> CGNKENASNGASGKNDEKKTEQAEEMTIKHQLGEAKVKKNPEKVVVFDFGVLDTLDKLGVKVTALPQMNVPKYLEKYKSSDYQNVGSLMEPDFEKLSEIKPDVIFISGRQANLYDKLKEIGPTVYIGIDTQHYWDSFTNNMKLIGQMFGKEKEVDEELANIEKQIEEVKTKAADKKALIILTTGGKVSAYGKGSRFGLIHDVLGVPAADPNLKVTNPHGQSVSFEYIAEKNPDYLFVIDRDAVVEGKPTAKQTIENALVKKTKAYQNGHIVYLDPNYWYLSGGGLTSVSEMIKQVEEGLK

Siderophore-binding proteins from two thermophilic bacteria, Geobacillus stearothermophilus and Parageobacillus thermoglucosidasius, were identified from a search of sequence databases, cloned and overexpressed. They are homologues of the well characterized protein CjCeuE from Campylobacter jejuni. The proteins have a two-domain structure, with the domains linked by a long α-helix at the base of the fold. The siderophore binding sites sit between the two domains.

The crystal structure of apo Gst was solved by molecular replacement using the structure of CjCeuE as a search model. There is a single molecule in the asymmetric unit with a continuous chain from Met26 through to the C-terminal Lys300. The predicted and experimental apo Gst structures had an r.m.s.d. between all 273 Cα atoms of 0.62 Å. Thus, the AF2 model has accurately predicted the fold in the experimental apo structure around the ligand-binding site. In Gst and Pth, the position of the main chain of the histidine loop is closely similar in the apo, complex and predicted structures, with the histidine side chain having moved a couple of ångströms away from its iron-binding position in the apo and AF2 structures. In contrast, the histidine loop is already in the closed, iron-chelating position in the apo structures of the thermophilic proteins. It should of course be noted that these structures are from crystals cryogenically frozen at 100 K and that in natural Gst cells at their optimum growth temperature of around 65°C the His218 loop might well open up, as seen in CjCeuE. Apo Pth and Gst have a higher thermal unfolding transition midpoint (T m) and are substantially more thermostable than CjCeuE.> PISPIETVPVKLKPGMDGPKVKQWPLTEEKIKALVEICTEMEKEGKISKIGPENPYNTPVFAIKKKDSTKWRKLVDFRELNKRTQDFWEVQLGIPHPAGLKKKKSVTVLDVGDAYFSVPLDEDFRKYTAFTIPSINNETPGIRYQYNVLPQGWKGSPAIFQSSMTKILEPFKKQNPDIVIYQYMDDLYVGSDLEIGQHRTKIEELRQHLLRWGLTTPDKKHQKEPPFLWMGYELHPDKWTVQPIVLPEKDSWTVNDIQKLVGKLNWASQIYPGIKVRQLSKLLRGTKALTEVIPLTEEAELELAENREILKEPVHGVYYDPSKDLIAEIQKQGQGQWTYQIYQEPFKNLKTGKYARMRGAHTNDVKQLTEAVQKITTESIVIWGKTPKFKLPIQKETWETWWTEYWQATWIPEWEF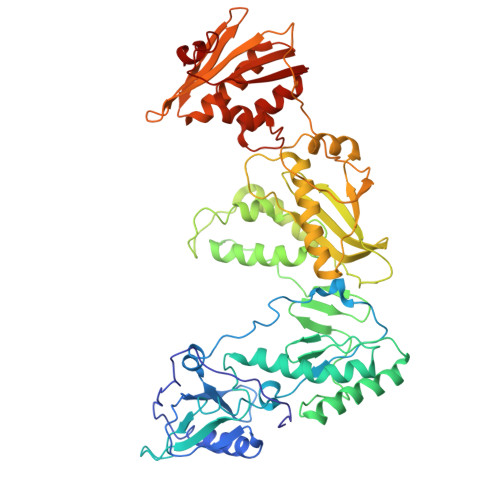VNTPPLVKLWYQLEKEPIVGAETFYVDGAANRETKLGKAGYVTNKGRQKVVPLTNTTNQKTELQAIYLALQDSGLEVNIVTDSQYALGIIQAQPDKSESELVNQIIEQLIKKEKVYLAWVPAHKGIGGNEQVDKLV(3R)-3-benzyl-4-[(4-methoxyphenyl)sulfonyl]-1-[(1-methyl-1H-imidazol-5-yl)methyl]-2,3,4,5-tetrahydro-1H-1,4-benzodiazepine-7-carbonitrile 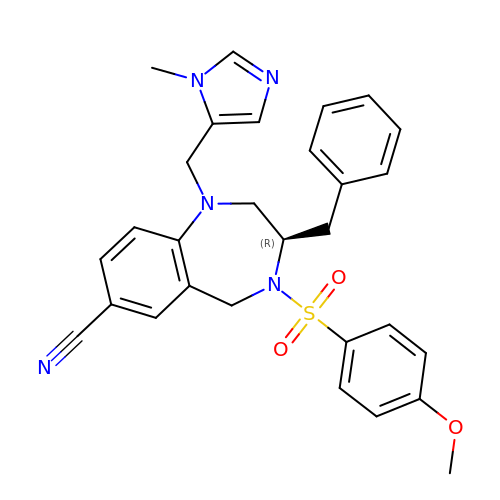| C29 H29 N5 O3 S | BJWZXDNEKWSGQH-RUZDIDTESA-N> MGLPPLLSLPSNSAPRSLGRVETPPEVVDFMVSLAEAPRGGRVLEPACAHGPFLRAFREAHGTAYRFVGVEIDPKALDLPPWAEGILADFLLWEPGEAFDLILGNPPYGIVGEASKYPIHVFKAVKDLYKKAFSTWKGKYNLYGAFLEKAVRLLKPGGVLVFVVPATWLVLEDFALLREFLAREGK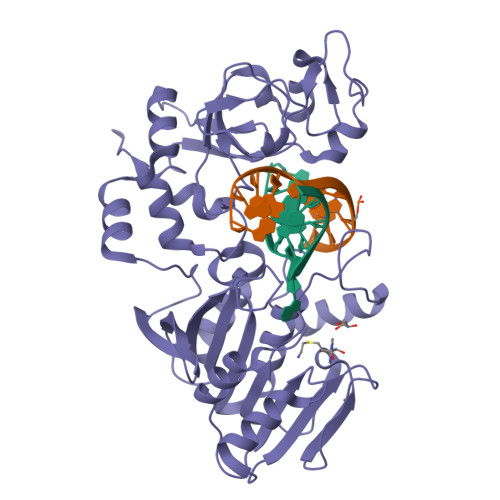TSVYYLGEVFPQKKVSAVVIRFQKSGKGLSLWDTQESESGFTPILWAEYPHWEGEIIRFETEETRKLEISGMPLGDLFHIRFAARSPEFKKHPAVRKEPGPGLVPVLTGRNLKPGWVDYEKNHSGLWMPKERAKELRDFYATPHLVVAHTKGTRVVAAWDERAYPWREEFHLLPKEGVRLDPSSLVQWLNSEAMQKHVRTLYRDFVPHLTLRMLERLPVRREYGFHTSPESARNF> MKKLILLTLIIASFDIYAI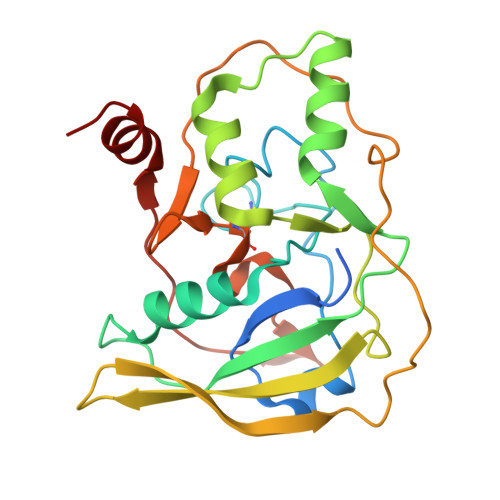DFVYRVDPNPPDVIFRDGFSLLGYNRDLQQLISGRSCAGGSSDSRYIVTTSDINKTYAIARAYYSHSKFKGNLYRYKIRADNNFYSLTPSVNYLESQGGHFNAYEKSMIRLQSEYVSTLSILPENIQKAVALVYDSSTGQIKDGTSTINTDYVSISSVSNPGVIPFLPEPQANTQQRIDAFGSLISSCFSIYSVCQTHRGQKTEVYKMPFYDARPVIQFIISGN>[4x]MSAVFGAKYTLRFGHVLAPGEPYHQAFLKWAKAVEEKTNGDVRIEVFPSSQLGVEEDIIEQIRMGAPVGWNTDSARLGMYVKDIGVMNLAYFIDFMGAKTPEEAIEVLKKIKQSPTMQKWLKELEQRFGIKVLSFYWVQGYRHFVTNKPIRKPEDLNGLRIRTPGAPAWQESIRSLGAIPVAVNFGEIYTAVQTRAVDGAELTYANVYNGGLYEVLKYMSETGHFLLINFEIVSADWF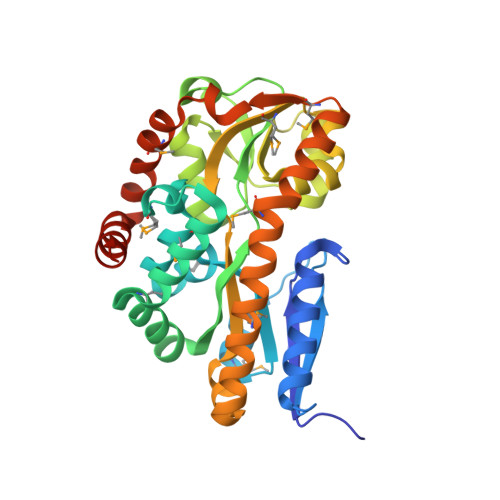NSLPKEYQKIIEEEMDKAGIEVSLKIMKELEEEYKQKCIEKGMAVIPASEIDKEAFMEKAKQAYKNLGLENALNQLIKEVKGEHHHHHH>MNSQLTLRALERGDLRFIHNLNNNRNIMSYWFEEPYESFDELEELYNKHIHDNAERRFVVEDAQKNLIGLVELIEINYIHRSAEFQIIIAPEHQGKGFARTLINRALDYSFTILNLHKIYLHVAVENPKAVHLYEECGFVEEGHLVEEFFINGRYQDVKRMYILQSKYLNRSE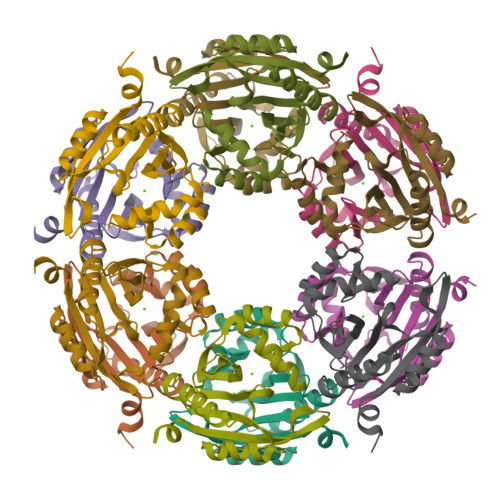[6x]>MPPLSLLIKPASSGCNLKCTYCFYHSLSDNRNVKSYGIMRDEVLESMVKRVLNEANGHCSFAFQGGEPTLAGLEFFEKLMELQRKHNYKNLKIYNSLQTNGTLIDESWAKFLSENKFLVGLSMDGPKEIHNLNRKDCCGLDTFSKVERAAELFKKYKVEFNILCVVTSNTARHVNKVYKYFKEKDFKFLQFINCLDPLYEEKGKYNYSLKPKDYTKFLKNLFDFWYEDFLNGNRVSIRYFDGLLETILLGKSSSCGMNGTCTCQFVVESDGSVYPCDFYVLDKWRLGNIQDMTMKELFETNKNHEFIKLSFKVHEECKKCKWFRLCKGGCRRCRDSKED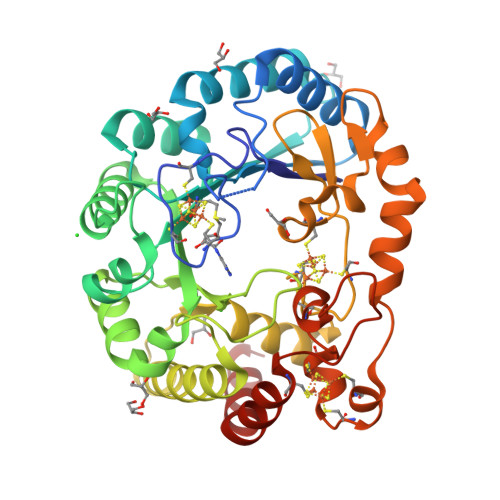SALELNYYCQSYKEFFEYAFPRLINVANNIK[2x]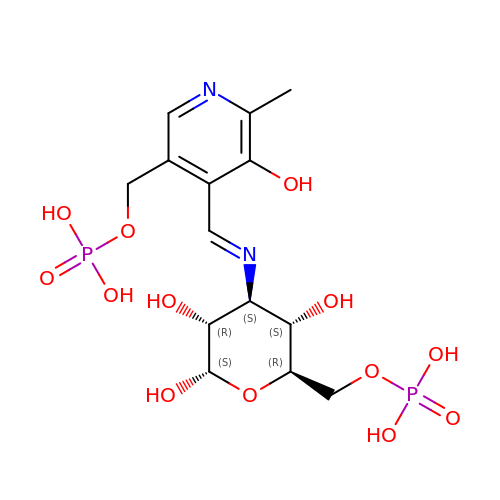3-deoxy-3-[(E)-({3-hydroxy-2-methyl-5-[(phosphonooxy)methyl]pyridin-4-yl}methylidene)amino]-6-O-phosphono-alpha-D-gluco pyranose | C14 H22 N2 O13 P2 | QZSIYKBKRPMGJB-ZKLPQXMUSA-N> ETGASVEGDNCEVKDPRHGNLYDLKPLGLNDTIVSAGEYTYYFRVCGKLSSDVCPTSDKSKVVSSCQEKREPQGFHKVAGLLTQKLTYENGLLKMNFTGGDTCHKVYQRSTAIFFYCDRGTQRPVFLKETSDCSYLFEWRTQYACPPFDLTECSFKDGAGNSFDLSSLSRYSDNWEAITGTGDPEHYLINVCKSLAPQAGTEP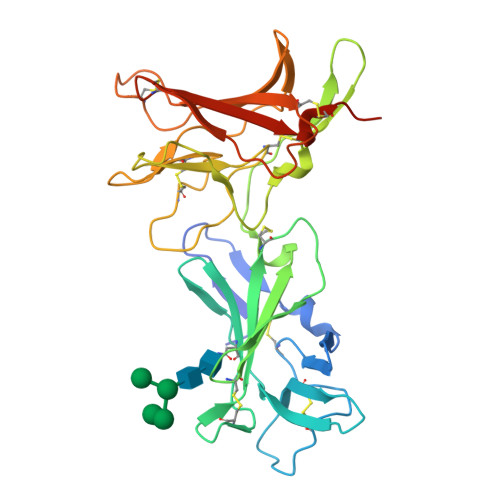CPPEAAACLLGGSKPVNLGRVRDGPQWRDGIIVLKYVDGDLCPDGIRKKSTTIRFTCSESQVNSRPMFISAVEDCEYTFAWPTATACPMKSTRHHHHHH GDP-N-acetylperosamine 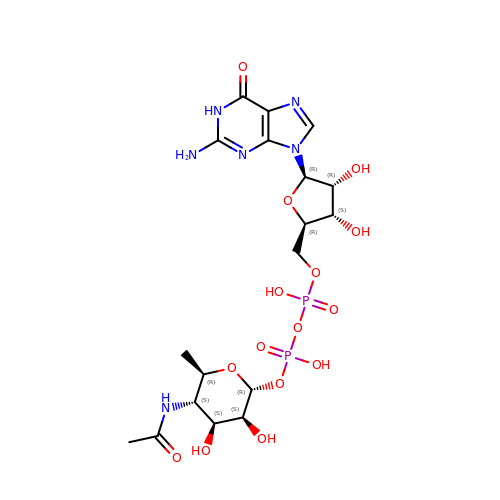| C18 H28 N6 O15 P2 | QYYLCPNKZRMSFL-XEDXKBCUSA-N> GSSGSSGMIKEYRTIKEVVGPLMAVEKVSGVKYEELIEVRMQNGEIRRGQVLEVQEDKAMVQIFEGTSGINYKNSSVRFLGHPLQLGVSEDMIGRVFDGLGRPKDNGPEILPEKYLDINGEVINPIARDYPDEFIQTGISAIDHLNTLVRGQKLPVFSGSGLPHKELAAQIARQATVLDSSDDFAVVFAAIGITFEEAEFFMEDFRQTGAIDRSVMFMNLANDPAIERIATPRMALTAAEYLAYEKGMHVLVIMTDMTNYAEALREISAARREVPGRRGYPGYLYTNLATLFERAGRIRGLKGSVTQIPILTMPEDDKTHPIPDLTGYITEGQIILTRELYKSGIQPPIDVLP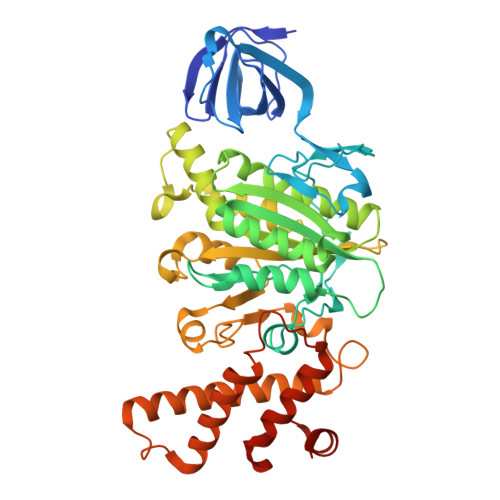SLSRLKDKGTGAGKTREDHAATMNQLFAAYAQGKQAKELAVVLGESALSDIDKIYAKFAERFENEYVNQGFYTNRTITETLDLGWELLAMLPRTELKRIKDDLLDKYLPEGK> MSTATARRRVVLTGFGVISSIGTGVEEYTAGLRAGRSGARPITRFDTEGFGQNTACEVPDFEPGRWIHHVPLDDMGRAGQYAVAAARMAVDDAGLTEDDLGERQAVITVGTTDGESHDIAVLLEQELAAGDPEAMDPVLARRINAGRLSTVIARELRMPNVEATTVTTACAAGNYSVGYGLDSIRSGEVDIALCGGADAVCRKAFALFKRFGALTPDVVRPFDKDRQGILTGEGAGILVLESLESALARG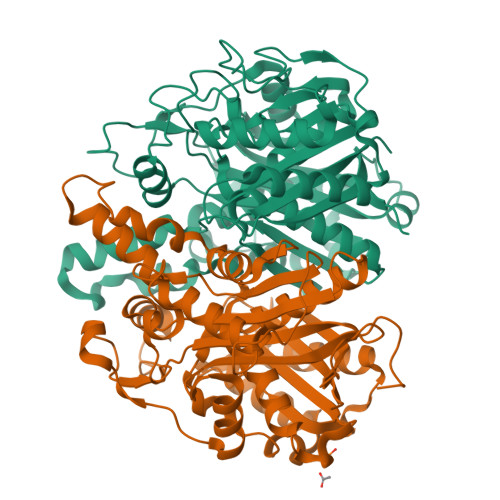ARIHAEVLGYGLSCDAAHPTAPNRDGIARGIRLALDDAGVEQEEIDFISAHGTGTKANDKTESAAIVDVYGDAPPRTVAVKSMLGHSMGAASALGAIACGLAIEHGFIPPTINHRETDPDCPLDVVPNRAVEADVRIVQNNSSAFAGNNAVLILGTYGE;> MTTMSTATARPEATLPPGTPVITGWSAVSPYGIGRAEFAAGVRAGAKTAVKADAGLGPLPSSDVCTVPGFDIQEQLGPRGTAKMDRLTALALVASDGLLLDADGNRAVATDELTGVVLGITMGSLENVTDFLRQSYTNARPFYVDAGRIPFGSLNHAAGATAIRHDLKGPNTTVAGGRVSGLLALNYARRLMGQGRATKYLVGSAEEFSAAHAWFEHTATASGDPAPLLGEGCGLFLVEQAEAAERPPLAAVLSVETRVDIDDDPGAAVTACARRALRRAGVDAGEVWAAVPCAAPTAAGRAEHEALAALVPADALSRVPSMELLGDTGAASASFQIAAVLAAAEADADSRGRIALVCAVDRDGAVAVAVLRLIGEQR> MYERFTDRARRVVVLAQEEARMLNHNYIGTEHILLGLIHEGEGVAAKSLESLGISLEGVRSQVEEIIGQGQQAPSGHIPFTPRAKKVLELSLREALQLGHNYIGTEHILLGLIREGE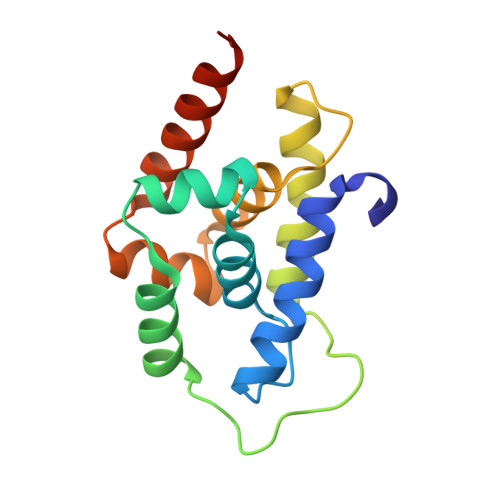GVAAQVLVKLGAELTRVRQQVIQLLSGYLEHHHHHH>GGVFPNVTNINSDKLLGGLLASGFDEDSCLSRYQSVHYRKPSPYKPSSYLISKLRNYEKLHKRCGPGTESYKKALKQLDQEHIDGDGECKYVVWISFSGLGNRILSLASVFLYALLTDRVLLVDRGKDMDDLFCEPFLGMSWLLPLDFPMTDQFDGLNQESSRCYGYMVKNQVIDTEGTLSHLYLHLVHDYGDHDKMFFCEGDQTFIGKVPWLIVKTDNYFVPSLWLIPGFDDELNKLFPQKATVFHHLGRYLFHPTNQVWGLVTRYYEAYLSHADE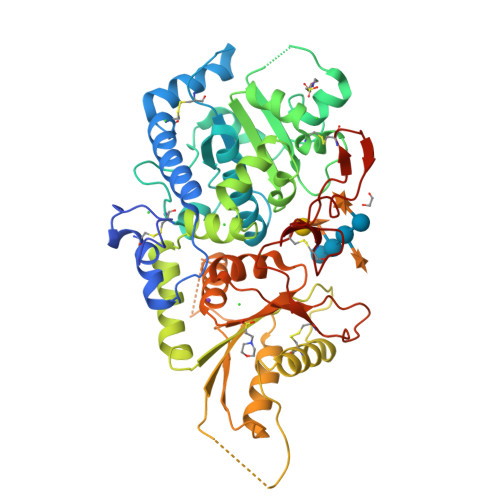KIGIQVRVFDEDPGPFQHVMDQISSCTQKEKLLPEVDTLVERSRHVNTPKHKAVLVTSLNAGYAENLKSMYWEYPTSTGEIIGVHQPSQEGYQQTEKKMHNGKALAEMYLLSLTDNLVTSAWSTFGYVAQGLGGLKPWILYRPENRTTPDPSCGRAMSMEPCFHSPPFYDCKAKTGIDTGTLVPHVRHCEDISWGLKLV[4x]The tri-longin domain (TLD) RabGEF complexes represent a family of RabGEFs with a unique conserved structural core. In each complex, two subunits that contain three longin domains (LD1 to LD3) each form a heterodimer, which is required for catalytic activity toward the cognate Rab GTPases. We here report the cryo-EM structures of the Mon1-Ccz1 and Inturned-Fuzzy core complexes bound to their cognate GTPases Ypt7 and Rab23 in the nucleotide exchange transition states, revealing a conserved catalytic mechanism with distinct modes of substrate recognition. Thus, TLD RabGEFs rely on both conservation and variability in the switch 1 regions of their substrates to realize catalytic efficiency and specificity.

Last, the TLD proteins Fuzzy and Inturned act as GEF for Rab23 (5). All longin domains of Fuzzy and Inturned are well resolved, but as in CPLANE, an N-terminal PDZ domain of Inturned is not visible in the map. However, analysis of the surface properties of the Fuzzy-Inturned complex reveals a mixed distribution of positive and negative charges and no conserved basic or hydrophobic patches. Fuzzy-Inturned does bind neither liposomes generated from a neutral lipid mix that has few packing defects (PO) nor charged liposomes with increased packing defects (DO/PIP/PS). We also could not detect any interaction of Fuzzy-Inturned with liposomes that have a high content of 5% PI3P. Our findings are not consistent with the previously suggested function of Inturned and Fuzzy as PIP-binding proteins, pointing to alternative mechanisms. Thus, the Fuzzy-Inturned complex may also be localized to its target compartments by interactions with recruiter proteins that enable tight membrane binding. Furthermore, Fuzzy-Inturned could be recruited to the liposomes by CiBAR1 and Rsg1 but not by Rsg1 alone. Thus, CiBAR1 serves as an adaptor protein for the mammalian CPLANE complex.

> VGEEGTGGTVHLLCLAASSGVPLFCRSSRGGAPARQQLPFSVIGSLNGVHMFGQNLEVQLSSARTENTTVVWKSFHDSITLIVLSSEVGISELRLERLLQMVFGAMVLLVGLEELTNIRNVERLKKDLRASYCLIDSFLGDSELIGDLTQCVDCVIPPEGSLLQEALSGFAEAAGTTFVSLVVSGRVVAATEGWWRLGTPEAVLLPWLVGSLPPQTARDYPVYLPHGSPTVPHRLLTLTLLPSLELCLLCGPSPPLSQLYPQLLERWWQPLLDPLRACLPLGPRALPSGFPLHTDILGLLLLHLELKRCLFTVEPLGDKEPSPEQRRRLLRNFYTLVTSTHFPPEPGPPEKTEDEVYQAQLPRACYLVLGTEEPGTGVRLVALQLGLRRLLLLLSPQSPTHGLRSLATHTLHALTPLL;> MDYKDDDDKGVPRIPMASVASCDSRPSSDELPGDPSSQEEDEDYDFEDRVSDSGSYSSASSDYDDLEPEWLDSVQKNGELFYLELSEDEEESLLPETPTVNHVRFSENEIIIEDDYKERKKYEPKLKQFTKILRRKRLLPKRCNKKNSNDNGPVSILKHQSNQKTGVIVQQRYKDVNVYVNPKKLTVIKAKEQLKLLEVLVGIIHQTKWSWRRTGKQGDGERLVVHGLLPGGSAMKSGQVLIGDVLVAVNDVDVTTENIERVLSCIPGPMQVKLTFENAYDVKRETSHPRQKKTQSNTSDLVKLLWGEEVEGIQQSGLNTPHIIMYLTLQLDSETSKEEQEILYHYPMSEASQKLKSVRGIFLTLCDMLENVTGTQVTSSSLLLNGKQIHVAYWKESDKLLLIGLPAEEVPLPRLRNMIENVIQTLKFMYGSLDSAFCQIENVPRLDHFFNLFFQRALQPAKLHSSASPSAQQYDASSAVLLDNLPGVRWLTLPLEIKMELDMALSDLEAADFAELSEDYYDMRRLYTILGSSLFYKGYLICSHLPKDDLIDIAVYCRHYCLLPLAAKQRIGQLIIWREVFPQHHLRPLADSSTEVFPEPEGRYFLLVVGLKHYMLCVLLEAGGCASKAIGSPGPDCVYVDQVKTTLHQLDGVDSRIDERLASSPVPCLSCADWFLTGSREKTDSLTTSPILSRLQGTSKVATSPTCRRTLFGDYSLKTRKPSPSCSSGGSDNGCEGGEDDGFSPHTTPDAVRKQRESQGSDGLEESGTLLKVTKKKSTLPNPFHLGNLKKDLPEKELEIYNTVKLTSGPENTLFHYVALETVQGIFITPTLEEVAQLSGSIHPQLIKNFHQCCLSIRAVFQQTLVEEKKKGLNSGDHSDSAKSVSSLNPVKEHGVLFECSPGNWTDQKKAPPVMAYWVVGRLFLHPKPQELYVCFHDSVTEIAIEIAFKLFFGLTL> GAMERVLKVFHYFENSSEPTTWASIIRHGDATDVRGIIQKIVDCHKVKNVACYGLRLSHLQSEEVHWLHLDMGVSNVREKFELAHPPEEWKYELRIRYLPKGFLNQFTEDKPTLNFFYQQVKNDYMLEIADQVDQEIALKLGCLEIRRSYGEMRGNALEKKSNYEVLEKDVGLRRFFPKSLLDSVKAKTLRKLIQQTFRQFANLNREESILKFFEILSPVYRFDKECFKCALGSSWIISVELAIGPEEGISYLTDKGANPTHLADFNQVQTIQYSNSEDKDRKGMLQ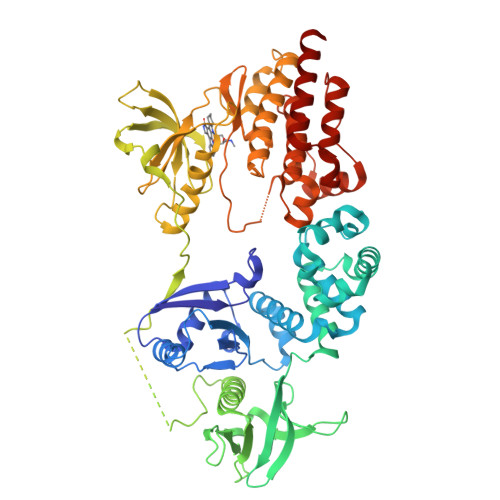LKIAGAPEPLTVTAPSLTIAENMADLIDGYCRLVNGATQSFIIRPQKEGERALPSIPKLANNEKQGVRSHTVSVSETDDYAEIIDEEDTYTMPSTRDYEIQRERIELGRCIGEGQFGDVHQGIYMSPENPAMAVAIKTCKNCTSDSVREKFLQEALTMRQFDHPHIVKLIGVITENPVWIIMELCTLGELRSFLQVRKFSLDLASLILYAYQLSTALAYLESKRFVHRDIAARNVLVSSNDCVKLGDFGLSRYMEDSTYYKASKGKLPIKWMAPESINFRRFTSASDVWMFGVCMWEILMHGVKPFQGVKNNDVIGRIENGERLPMPPNCPPTLYSLMTKCWAYDPSRRPRFTELKAQLSTILEEEKLQ>[2x]MNSRMKIKKAYEYMKSFHQHDTTGHDIAHVERVYNNACYIAKRENITDTLVIELSSLLHDTVDSKLTDEILAYDQLK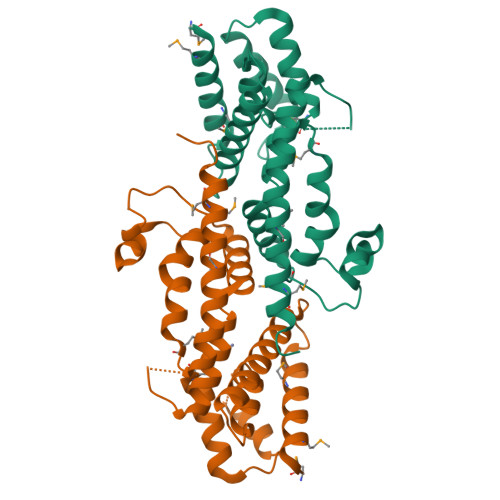QFLSTLDLSSEISQQVLYIIKHMSYRAGKNNHVKLSIDGEIVRDADRLDAIGAIGIARTFQFSGHFGEPMWTETKLSNEELHTSLVEELDNSAIKHFYEKLFKLKDLMHTPTAKKLAEERHQFMIQYLKQFMSEWNFNKELEHHHHHH>MSRFIRASQRRTLLATLIAATLAQPLLAAESLDSKPASAITAAKNAEVLKNLPFADREEFEAAKRGLIAPFSGQIKNAEGQVVWDMGAYQFLNDKDAADTVNPSLWRQAQLNNIAGLFEVMPKLYQVRGLDPANMTIIEGDSGLVLIDTLTTAETARAALDLYFQHRPKKPIVAVVYSHSHIDHFGGARGIIDEADVKAGKVKVFAPSGFMEHAVSENILAGTAMARRGQYQSGVMV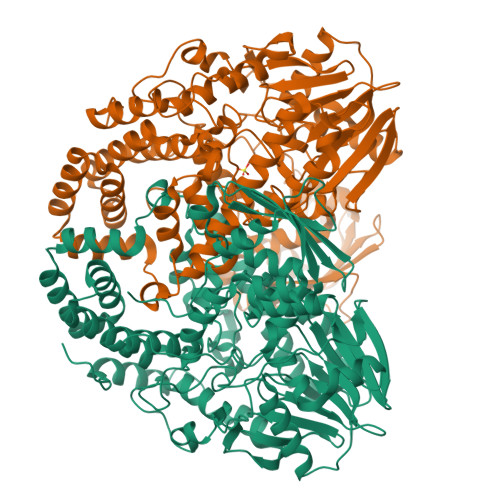PRGAQAQVDSGLFKTTATNATNTLVAPNVLIEKPYERHTVDGVELEFQLTLGSEAPSDMNIYLPQFKVLNTADNAPPAMHNLLTPRGAEVRDAKAWAGYIDASLEKYGDRTDVLIQQHNWPVWGGDKVRTYLADQRDMYAFLNNRALNLMNKGLTLHEIAAEVSKLPGELDRKWYLRSYYGALSTNLRAVYQRYLGFYDGNPANLDPFPPVEAGKRYVEAMGGADAVLKQMRAAIDKGDYRWAVQLGNHLVFADPANKDARALQADAMEQLGYQTENALWRNMYMTGAMELRHGVPTYDSRGKSEMGRALTPDMFFDLLAIRLDTDKAVGHDMTLNWVFEDLKQDIALTLRNGVLTQRVGSLNPKADVTVKLTKPTLDQIAARKLDLPTAIKQGTVKLDGDGKKLGEFFGLLDSFSPKFNIVELEHHHHHH[2x]>[12x]MRGSHHHHHHGSTSSSTPRHRGIFPVVPTTFADTGELDLASQ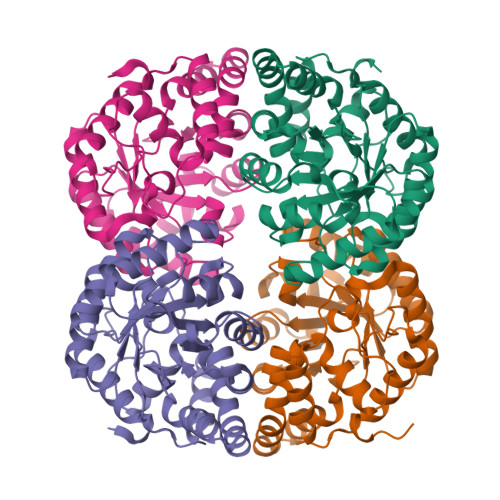KRAVDFMIDAGSDGLCILANFSEQFAITDDERDVLTRTILEHVAGRVPVIVTTSHYSTQVCAARSLRAQQLGAAMVMAMPPYHGATFRVPEAQIFEFYARVSDAIAIPIMVQDAPASGTALSAPFLARMAREIEQVAYFKIETPGAANKLRELIRLGGDAIEGPWDGEEAITLLADLHAGATGAMTGGGFPDGIRPILEAWREGRHDDAYARYQAWLPLINHENRQSGILTAKALMREGGVIASERPRHPMPELHPDTRAELLAIARRLDPLVLRWAH>[6x]MNHKVHHHHHHIEGRHMALAAPPGELTLALTPDDKTLDPASLDRALAILAEHGILVLTGMLRTRLTDQLRTAMLDDLPEVLRQQDVPTNFVPGHVQQDPPVRESLLFPDVLLNPVVYQITHAVLGADARNAVYSGNMNLPGSHEQPVHLDEPHLWPGISHPPYCLCVDVPLIDFTLENGSTEYWPGSHVLNPDECYDERGCVLPAELER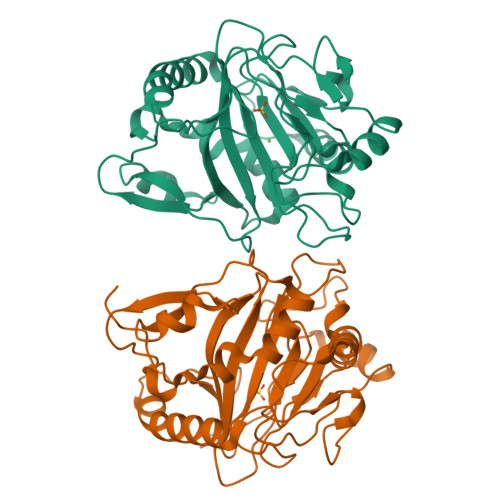RRAVAPPVRFPIPVGSVVIRDGRLWHRGVPNLSAAPRPLLAMTHYTEWFDMPPIQLPDTVKSWVDGSDRHTHAHFVAGDVDHLTGDHPFAVR> MNNNEPDTLPDPAIGYIFQNDIVALKQAFSLPDIDYADISQREQLA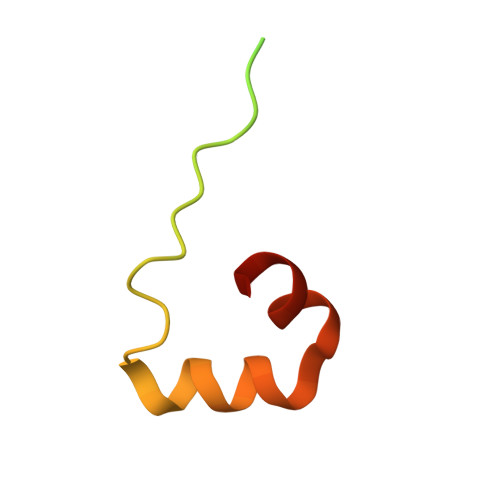AALKRWPLLAEFAQQK> CUGGGUCGCAGUNNCCCCAG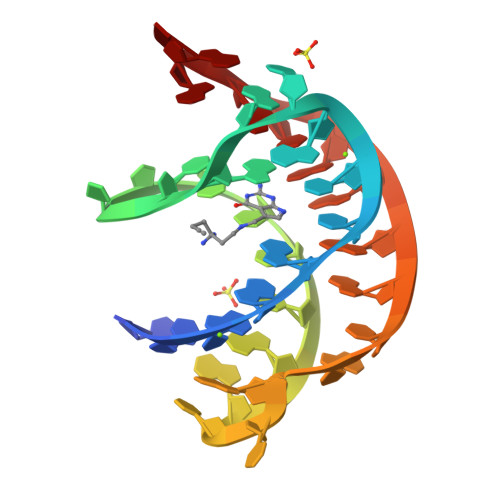UUAACAAAACAAG>GIDPFTMVSVDNTYQSLERELANDDPWRLDDNPFERERHTQLLRLSLSSGAVSNGLEIGCAAGAFTEKLAPHCKRLTVIDVMPRAIGRACQRTKRWSHISWAATDILQFSTAELFDLIVVAEVLYYLE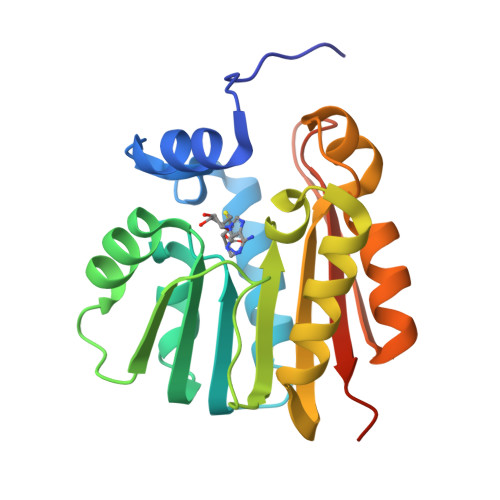DMTQMRTAIDNMVKMLAPGGHLVFGSARDATCRRWGHVAGAETVITILTEALTEVERVQCQGQSADEDCLLARFRNPERSSIRPDGRA[4x]13(R)-HYDROPEROXY-9(Z),11(E)-OCTADECADIENOIC ACID | C18 H32 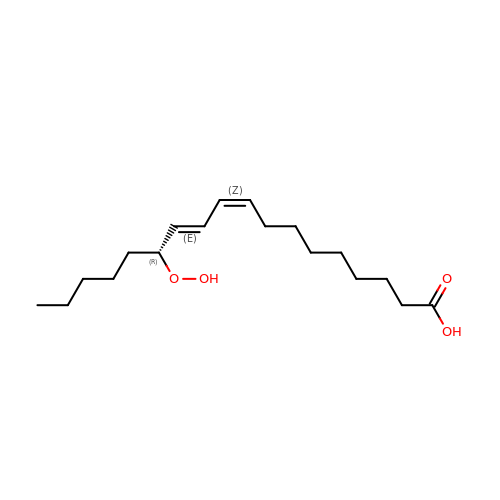O4 | JDSRHVWSAMTSSN-PIHGWCCBSA-N>GSQQLTYSQLVLRTAIQDQYSKLSGDGPFPMAFGLVLSEEERREVIDLYSLQFQYPDQPELQRLVILPQTHSTRTRRRAKGSYTWYLRS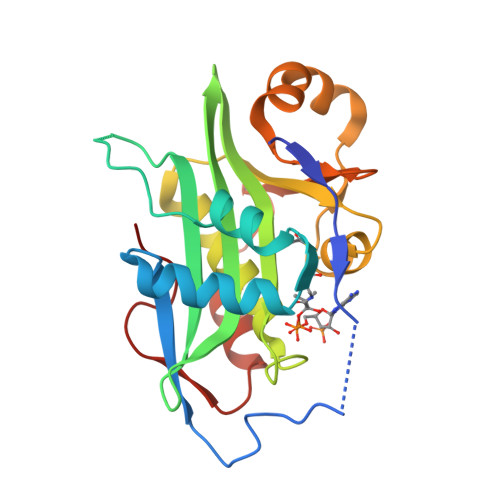LNTNEMVCAVTIMAHHYETHHFVEVPLFATGVGYKKHGFGRLMNAALLQWCVETGFEFVMISADVKAIPFWSHLGYKTMEKSELTRIVFYYEHNCYKFKGAEVMIRYCRTWPTDGVKEALARVQKVIVSGHVGLMDA[2x]In cyanobacteria, carotenoid-dependent non-photochemical quenching is mediated by a unique class of water-soluble carotenoid-binding proteins, the homologs of the Orange Carotenoid Protein (OCP). In the compact dark-adapted orange state (OCPO), the ketocarotenoid is enclosed by two protein domains of about equal size: an all α-helical N-terminal domain (NTD) and a mixed α-helical/β-sheet C-terminal domain (CTD). Upon photoactivation, OCP converts into the physiologically active red state (OCPR) via the formation of numerous intermediates, and the quantum yield of OCPR formation is extremely low (about 0.2%). ICT signatures are valuable indicators for the contribution of the carbonyl group(s) to the conjugated system, and might inform on the configuration of the carotenoid end rings. These effects are of particular interest for the chromophores embedded in OCP since the only specific carotenoid-protein interactions in the OCPO state are two short and strong hydrogen bonds between the 4-keto oxygen of the carotenoid and two hydrogens in the CTD, one belonging to the Tyr-201 hydroxyl group and another to the N-H group of Trp-288 (numbering corresponds to the OCP sequence of Synechocystis sp. PCC 6803).

A 1.37 Å crystal structure of OCP Y201W combined with femtosecond time-resolved absorption spectroscopy, kinetic analysis, and deconvolution of the spectral intermediates, as well as extensive quantum chemical calculations incorporating the effect of the local electric field, highlighted the role of charge-transfer states during OCP photoconversion. To elucidate possible reasons behind the spectral heterogeneity of OCP in its compact orange state, we determined the atomic structure of OCPWW. It crystallized at three different pH values in the same space group P3221, giving three structures with resolutions from 1.37 Å (pH 6.5) to 1.49 Å (pH 5.5). The position and conformation of Trp-288 are identical in WT and OCPWW, indicating the presence of a strong hydrogen bond between the keto oxygen and Trp-288 (the distance between the carotenoid’s keto oxygen and the nitrogen of Trp-288 is 2.9 Å). The electron density for the residue 201 reveals two alternative conformations of the engineered Trp in this position with nearly identical occupancies, nicely supported at this high level of spatial resolution. One Trp-201 conformation has the nitrogen oriented towards the keto group of the carotenoid (‘IN’ conformation), presumably enabling the formation of a weaker hydrogen bond with a distance of 3.2 Å. In the second Trp-201 conformation (‘OUT’), the side chain is rotated by 180° roughly in the same plane, which is incompatible with a hydrogen bond to the keto oxygen of ECN. Analysis of Fo-Fo difference maps shows that IN and OUT Trp-201 rotamers have identical occupancy (within experimental error) each at all probed pHs.

> MRGSHHHHHHTDPATMPFTIDSARGIFPNTLAADVVPATIARFSQLNAEDQLALIWFAYLEMGKTLTIAAPGAASMQLAENALKEIQAMGPLQQTQAMCDLANRADTPLCRTYASWSPNIKLGFWYRLGELMEQGFVAPIPAGYQLSANANAVLATIQGLESGQQITVLRNAVVDMGFTAGKDGKRIAEPVVPPQDTASRTKVSIEGVTNATVLNWMDNLNANDFDTLIELFTSDGALQPPFQRPIVGKENVLRFFREECQNLKLIPERGVTEPAEDGFTQIKVTGKVQTPWFGGNVGMNIAWRFLLNPEGKIFFVAIDLLASPKELLNFAR1,5-anhydro-2-{[5-(2-chloro-4-phenoxybenzene-1-carbonyl)-7H-pyrrolo[2,3-d]pyrimidin-4-yl]amino}-2,3,4-trideoxy-D-erythro-hexitol | C25 H23 Cl N4 O4 | 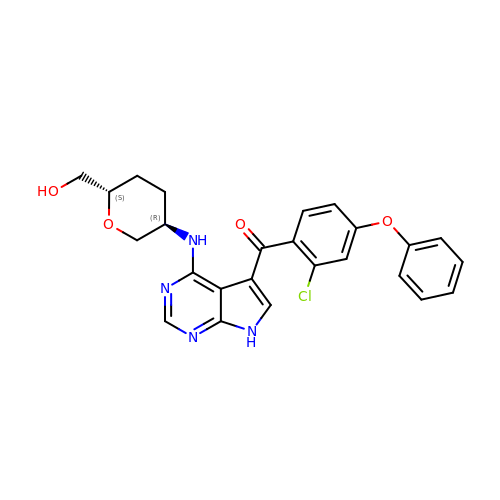JSFCZQSJQXFJDS-QAPCUYQASA-N> GHMERLLDELTLEGVARYMQSERCRRVICLVGAGISTSAGIPDFRSPSTGLYDNLEKYHLPYPEAIFEISYFKKHPEPFFALAKELYPGQFKPTICHYFMRLLKDKGLLLRCYTQNIDTLERIAGLEQEDLVEAHGTFYTSHCVSASCRHEYPLSWMKEKIFSEVTPKCEDCQSLVKPDIVFFGESLPARFFSCMQSDFLKVDLLLVMGTSLQVQPFASLISKAPLSTPRLLINKEKAGQSDPFLGMIMGLGGGMDFDSKKAYRDVAWLGECDQGCLALAELLGWKKELEDLVRREHASIDAQS;> EALPKATGG

Sirtuins (SIRTs) are nicotinamide adenine dinucleotide (NAD+)‐dependent lysine deacylases linked to key physiological and disease processes. SIRTs catalyze lysine deacylation through a distinctive mechanism in which the amide oxygen of the acylated lysine transiently attacks the C1’ of the nicotinamide riboside residue from NAD+ (hereafter referred to as C1’ of NAD+ ribose), forming a covalent ADP‐ribosylated intermediate. Here, we report a new class of mechanism‐based 1,2,3‐triazole inhibitors that hijack SIRT catalysis by forming stalled triazolium– or triazole–ADP‐ribose (ADPR) adducts derived from the cofactor NAD+. These trapped adducts inhibit the enzyme without covalent protein modification, prompting us to term the compounds “Sirtuin Trapping Ligands” (SirTraps).

Compounds OTi‐1 (3, ornithine‐triazolyl inhibitor 1) and LTi‐1 (4, lysine‐triazolyl inhibitor 1) mimic acetylated lysine (Kac), whereas OTDi‐1 (5, ornithine‐triazolyl‐dodecyl inhibitor 1) and LTDi‐1 (6, lysine‐triazolyl‐dodecyl inhibitor 1) mimic Kmyr through their dodecyl extensions, engaging the full acyl‐lysine channel. To elucidate the molecular basis of this unexpected mode of inhibition, co‐crystallization experiments were performed with SIRT2 and compounds 5 and 6, both in the absence and presence of NAD⁺. In contrast, significant melting temperature shifts were observed for 5 and 6 at 10 µM, further enhanced by NAD+ addition (ΔT m: 5 = 9.9 ± 0.0 °C, 6 = 16.3 ± 0.1 °C), indicating strong SIRT2 stabilization. Compound 6 exhibited an IC50 of 28 ± 6 nM, which was further reduced to 3.6  ± 0.6 nM after 15 min of NAD+ preincubation, implying cofactor‐assisted binding. Without NAD+, rapid dissociation was observed (k off = 7.1 × 10−3 ± 1.4 × 10−4 s−1), consistent with a fast on/off mechanism. Preincubation with NAD+ markedly slowed dissociation (k off = 2.6 × 10−4 ± 8.5 × 10−6 s−1), accounting for the high potency of compound 6.>QDNSRYTHFLTQHYDAKPQGRDDRYCESIMRRRGLTSPCKDINTFI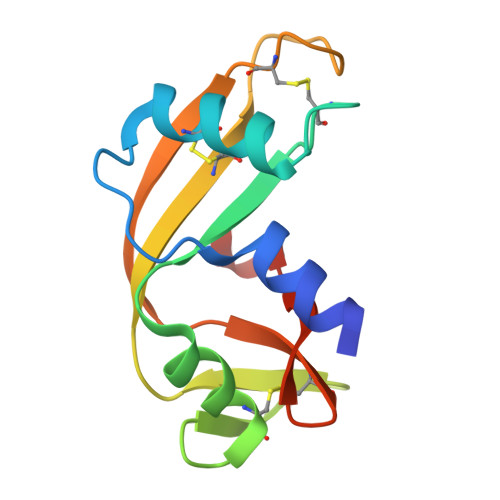HGNKRSIEAICENKNGNPHRENLRISKSSFQVTTCKLHGGSPWPPCQYRATAGFRNVVVACENGLPVHLDQSIFRRP[2x]> GSGIIKLRKEIERLEEKLEDANERIAELVKLEERQRIARDLHDTLGQKLSLIGLKSDLARKLIYKDPEQAARELKS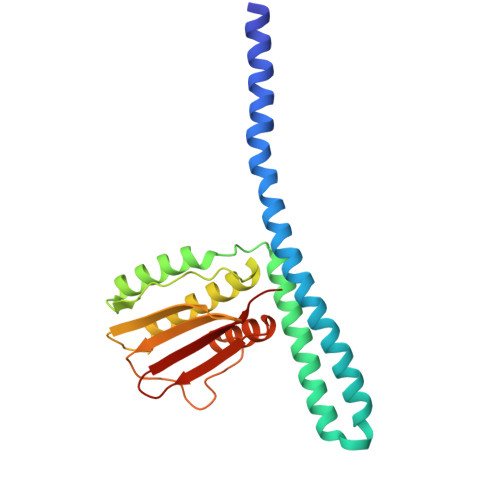VQQTARTSLNEVRKIVSSMKGIRLKDELINIKQILEAADIMFIYEEEKWPENISLLNENILSMCLKEAVTNVVKHSQAKTCRVDIQQLWKEVVITVSDDGTFKGEENSFSKGHGLLGMRERLEFANGSLHIDTENGTKLTMAIPNNSK OsSUF4 encodes a C2H2-type zinc finger transcription factor. OsSUF4 comprises two conserved C2H2-type zinc finger domains at the N-terminus and a large proline-rich domain at the C-terminus. OsSUF4 physically interacts with SDG725 and recognizes a 7-bp DNA element within the promoter regions of the rice florigen genes RICE FLOWERING LOCUS T1 (RFT1) and Heading date 3a (Hd3a) to promote rice flowering. The C-terminal domain of OsSUF4 interacts with SDG725 and the N-terminal zinc finger domain of OsSUF4 is responsible for DNA binding.

To unravel the structural basis underlying target DNA recognition by OsSUF4, we carried out a crystallographic study of the zinc finger domain (aa 10–100) of OsSUF4. The structure was solved by a Se-SAD phasing method and refined up to 1.95 Å resolution. The OsSUF4 zinc finger domain contained two C2H2 type zinc finger motifs with different folding. The first zinc finger motif adopts a canonical C2H2 fold containing a short antiparallel β-sheet followed by one α-helix; instead of a β-sheet, the second zinc finger motif contains a coiled-coil. The zinc-coordinating cysteines and histidines located in the β-sheet/coiled-coil and the α-helix, respectively, and coordination of the two zinc ions are very similar. In many known C2H2-type zinc finger proteins, neighboring C2H2 motifs are connected by long and flexible loops; however, only two residues were shown to be embedded in the junction region of the two zinc finger motifs of OsSUF4, preventing them from synchronously nestling into the DNA major groove. Notably, the first zinc finger domain is enriched with positively charged residues (R18, K24, K31, K33, K36, and K43), forming an electropositive interface. The wild-type OsSUF4 zinc finger domain bound to the substrate DNA (5′-GGGTACGGAAATGGTA-3′) with a Kd value of 51.28 ± 3.68 μM, whereas R18A, K24A, K31A, K33A, K36A, K43A, and R18A/K33A/K36A/K43A mutants all lost their DNA-binding ability. Compared with wild-type OsSUF4, Hd3a promoter activation by all single mutant proteins was significantly reduced; a more dramatic reduction was observed for the R18A/K33A/K36A/K43A mutant. Taken together, our findings suggested that the positive residues within the surface of the first zinc finger motif are essential for target DNA binding by OsSUF4.

> MGKKKKRVEKVFCYYCDREFDDEKILVQHQKAKHFKCHVCHKKLSTAGGMAIHVLQVHKESVTKVPNAKPERESTEIEIFGMQGIPPDVLAAHYGE[(2~{R},3~{S},4~{R},5~{R})-5-(6-aminopurin-9-yl)-3,4-bis(oxidanyl)oxolan-2-yl]methyl [(~{S})-azanyl-[[(5~{S},6~{E},8~{S},9~{S},12~{R},13~{E},15~{E})-21-chloranyl-12,20-dimethoxy-6,8,16-trimethyl-5-oxidanyl-3,11-bis(oxidanylidene)-2-azabicyclo[16.3.1]docosa-1(21),6,13,15,18(22),19-hexaen-9-yl]oxy]-oxidanyl-methyl] 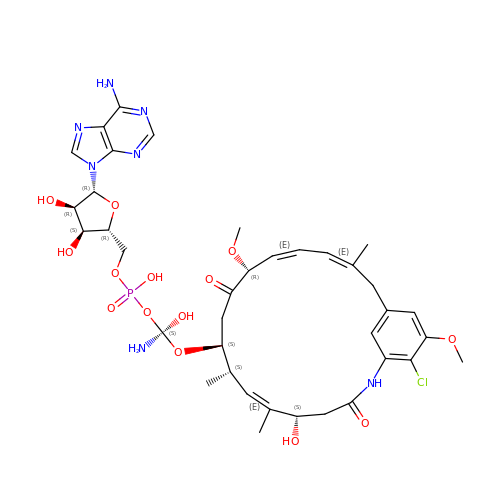hydrogen phosphate | C37 H49 Cl N7 O14 P | QLSIIXOKLGYKPW-VYDMNOPCSA-N> GGGGGPDYLYAEYRALPSPRQTGKNLRIGDGFSKYDNMTGVYLEKGRHVVLVGKTEGQEISLLLPNLMRKPAEGVQPTKDPNGWGLHKKQIPLKEGINIIDVETPANAYISYFTEDAGKAPKIPVHFVTGKANGYFDTTRGDTNKDWVRLLDQAVSPIMDARGKYIQVAYPVEFLKKFTKDRGTELINAYDKLIGIQYQLMGLDKYGKIP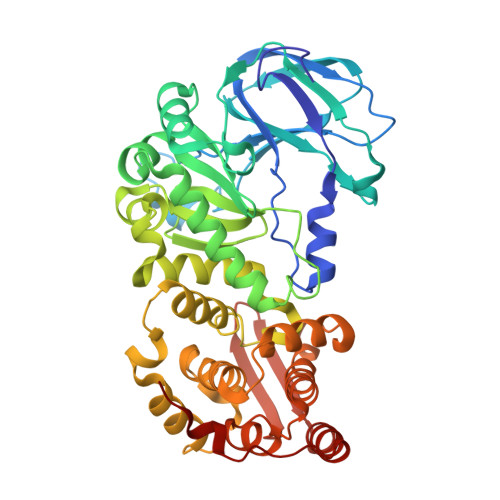ENRVLARVNFNYYMFRDGDGVAYLGNDGTMRMVTDPENVLKGDACWGFSHAVGHVMQMRPMTWGGMTEVSNNIFSLQAAAKTGNESRLKRQGSYDKARKEIIEGEIAYLQSKDVFNKLVPLWQLHLYFTKNGHPDFYPDVMEYLRNNAGNYGGNDTVKYQFEFVKACCDVTKTDLTDFFEKWGFFKPGKFHIGDYAQYDFNVTPEMVEETKKWIAGKGYPKPETDITELSE>HLPLIAITRNPVFPRFIKIIEVKNKKLVELLRRKVRLAQPYVGVFLKRDDSNESDVVESLDEIYHTGTFAQIHEMQDLGDKLRMIVMGHRRVHISRQLEVEPEEPEAENKHKPRRKSKRGKKEAEDELSARHPAELAMEPTPELPAEVLMVEVENVVHEDFQVTEEVKALTAEIVKTIRDIIALNPLYRESVLQMMQAGQRVVDNPIYLSDMGAALTGAESHELQDVLEETNIPKRLYKALSLLKKEFELSKLQQRLGREVEEKIKQTHRKYLLQEQLKIIKKELGLEKDDKDAIEEKFRERLKELVVPKHVMDVVDEELSKLGLLDNHSSEFNVTRNYLDWLTSIPWGKYSNENLDLARAQAVLEEDHYGMEDVKKRILEFIAVSQLRGSTQGKILCFYGPPGVGKTSIARSIARALNREYFRFSVGGMTDVAEIKGHRRTYVGAMPGKIIQCLKKTKTENPLILIDEVDKIGRGYQGDPSSALLELLDPEQNANFLDHYLDVPVDLSKVLFICTANVTDTIPEPLRDRMEMINVSGYVAQEKLAIAERYLVPQARALCGLDESKAKLSSDVLTLLIKQYCRESGVRNLQKQVEKVLRKSAYKIVSGEAESVEVTPENLQDFVGKPVFTVERMYDVTPPGVVMGLAWTAMGGSTLFVETSLRRPQDKDAKGDKDGSLEVTG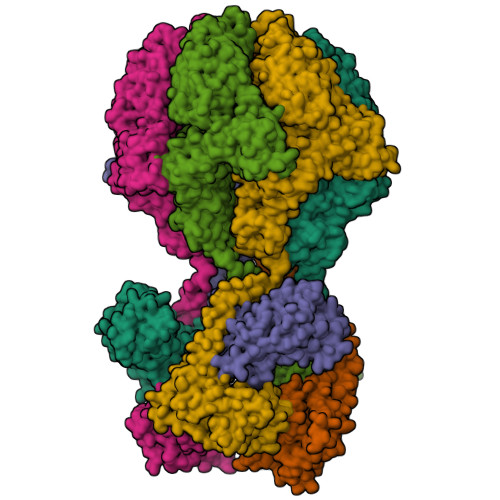QLGEVMKESARIAYTFARAFLMQHAPANDYLVTSHIHLHVPEGATPKDGPSAGCTIVTALLSLAMGRPVRQNLAMTGEVSLTGKILPVGGIKEKTIAAKRAGVTCIVLPAENKKDFYDLAAFITEGLEVHFVEHYREIFDIAFP[6x]> GAMGKVTHSIHIEKSDTAADTYGFSLSSVEEDGIRRLYVNSVKETGLASKKGLKAGDEILEINNRAADALNSSMLKDFLSQPSL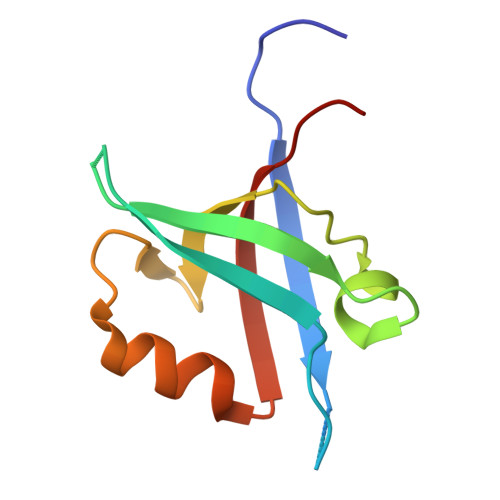GLLVRTYPEL>MKKEISVIGVPMDLGQMRRGVDMGPSAIRYAGVIERIEEIGYDVKDMGDICIEREKEIDENTKLRNLTQVATVCNELASKVDHIIEEGRFPLVLGGDHSIAIGTLAGVAKHYKNLGVIWYDAHGDLNTEETSPSGNIHGMSLAASLGYGHSSLVDLYGAYPKVKKENVVIIGARALDEGEKDFIRNEGIKVFSMHEIDRMGMTAVMEETIAYLSHTDGVHLSLDLDGLDPHDAPGVGTPVIGGLSYRESHLAMEMLAEADIITSAEFVEV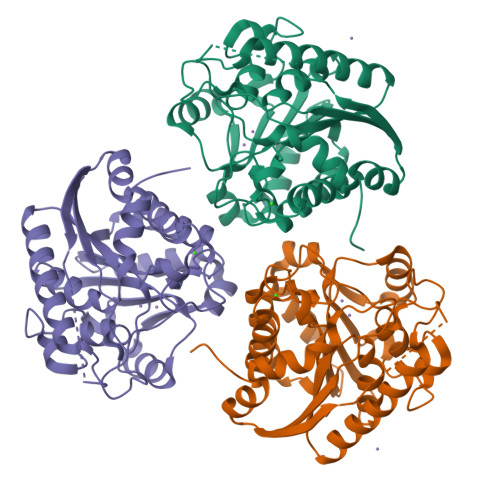NTILDERNRTATTAVALMGSLFGEKLK[6x]> MGSSHHHHHHSQGSMTPKLSKSLSFEMQQDELIEKPMSPMQYARSGLGTAEMNGKLIAAGGYNREECLRTVECYNPHTDHWSFLAPMRTPRARFQMAVLMGQLYVVGGSNGHSDDLSCGEMYDSNIDDWIPVPELRTNRCNAGVCALNGKLYIVGGSDPYGQKGLKNCDVFDPVTKLWTSCAPLNIRRHQS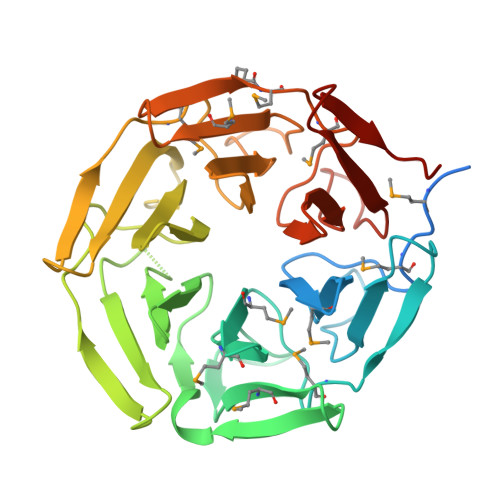AVCELGGYLYIIGGAESWNCLNTVERYNPENNTWTLIAPMNVARRGAGVAVLNGKLFVCGGFDGSHAISCVEMYDPTRNEWKMMGNMTSPRSNAGIATVGNTIYAVGGFDGNEFLNTVEVYNLESNEWSPYTKIFQF> HPPNRRGISFEVGAQLEARDRLKNWYPAHIEDIDYEEGKVLIHFKRWNHRYDEWFCW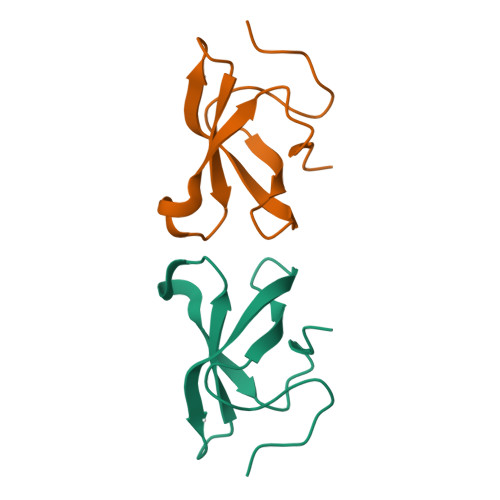DSPYLRPLE> SHVDPRIQGELEKLNQSTDDINRRETELEDARQKFRSVLVEATVKLDELVKKIGKAVEDSKPYWEARRVARQAQLEAQKATQDFQRATEVLRAAKETISLAEQRLLEDDKRQFDSAWQEMLNHATQRVAEAEQTKTRSELVHKETAARYNAAMGRMRQLEKKLKRAINKSKPYFELKAKYYVQLEQLKKTVDDLQAKLTLAKGEYKMALKNLEMISDEIHEAAASSAM

The Rab11 subfamily plays important roles in specific trafficking events such as exocytosis, endosomal recycling, and cytokinesis. SH3BP5 and SH3BP5-like (SH3BP5L) proteins have recently been found to serve as guanine nucleotide exchange factors (GEF) for Rab11. SH3BP5 exhibits a V-shaped structure comprising two coiled coils. The coiled coil composed of α1, and α4 is solely responsible for the Rab11a binding and GEF activity.

Because computational secondary structure prediction assigned the N- and C-terminal regions as mostly disordered regions, we selected the central helical region for crystallography. We found that the R260A/R261A/R262A triple mutation reduced the degradation and obtained diffraction-quality crystals. This construct of SH3BP5 (41–266; R260A/R261A/R262A) is hereafter referred to as SH3BP5-RA. In addition, the M167A mutation was introduced to improve the solubility of the selenomethionine (SeMet)-labeled SH3BP5-RA (SeMet SH3BP5-RA/M167A), which was used for phase determination by the single-wavelength anomalous diffraction method. Finally, we determined the crystal structures of SeMet SH3BP5-RA/M167A in two different crystal forms (I41 and P41) and native SH3BP5-RA at 3.35, 3.6, and 3.8 Å resolutions, respectively. The asymmetric units of the I41 and P41 crystals contain one and two SH3BP5 molecules, respectively. Therefore, we obtained five different apo-SH3BP5 structures in total (i.e., one from I41 SeMet SH3BP5-RA/M167A, two from P41 SeMet SH3BP5-RA/M167A, and two from P41 native SH3BP5-RA). Although these five apo-SH3BP5 structures exhibit a similar V-shaped conformation, the superposition of these five apo-SH3BP5 structures using α1 as the reference shows some flexibility of the conformation. The hinge region of the V shape contains staggered hydrophobic interactions so as to maintain the V shape.Two examples of protein crystals embedded in LCP were studied: lysozyme as a model soluble protein and a peptide transporter (PepTSt) as a more challenging membrane protein. Based on the obtained crystal coordinates, both still and rotation wedge serial data were collected automatically at the SLS PXI beamline, yielding in both cases a high indexing rate. We have produced an end-to-end demonstration of a simple yet robust and efficient offline crystal-prelocation method based on 2D full-field phase-contrast X-ray imaging on flat double-sandwich samples, a well established format for serial crystallography.

Crystal-specific properties such as the size and diffraction quality of individual crystals also influence the indexing process and therefore the measured overall efficiency. This could explain why the PepTSt samples yielded generally lower indexing rates than lysozyme. We attribute this difference to the crystal-quality variation between chip 1 and chip 2, as only chip 1 was used for rotation data collection. Such sample-to-sample variation is common for membrane-protein microcrystals. The prelocation method was successfully applied to both the conventional MX data collection with rotation method and still-image data collection by serial crystallography.

> MEDKGKTFFGQPLGLSTLFMTEMWERFSYYGMRAILLYYMWFLISTGDLHITRATAASIMAIYASMVYLSGTIGGFVADRIIGARPAVFWGGVLIMLGHIVLALPFGASALFGSIILIIIGTGFLKPNVSTLVGTLYDEHDRRRDAGFSIFVFGINLGAFIAPLIVGAAQEAAGYHVAFSLAAIGMFIGLLVYYFGGKKTLDPHYLRPTDPLAPEEVKPLLVKVSLAVAGFIAIIVVMNLVGWNSLPAYINLLTIVAIAIPVFYFAWMISSVKVTSTEHLRVVSYIPLFIAAVLFWAIEEQGSVVLATFAAERVDSSWFPVSWFQSLNPLFIMLYTPFFAWLWTAWKKNQPSSPTKFAVGLMFAGLSFLLMAIPGALYGTSGKVSPLWLVGSWALVILGEMLISPVGLSVTTKLAPKAFNSQMMSMWFLSSSVGSALNAQLVTLYNAKSEVAYFSYFGLGSVVLGIVLVFLSKRIQGLMQGVE>[2x]GPGSNATQINEELYRLLEDTEILNQEITEGLLKGFEVPDAGVAIQLSKRDVVYPARILIIVLSEMWRFGLTKQSESFLAQVLTTIQKVVTQLKGNDLIPSGVFWLANVRELYSFVVFALNS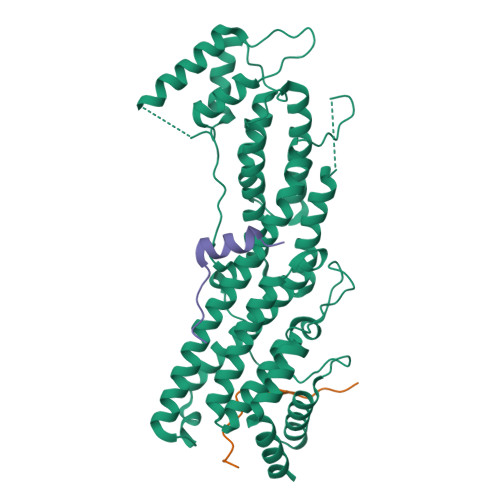ILTEETFKNGMTDEEYKEYVSLVTELKDDFEALSYNIYNIWLKKLQKQLQKKAINAVVISESLPGFSAGETSGANTEEYTMDDILTFFNSIYWCMKSFHIENEVFHAVVTTLLNYVDAICFNELIMKRNFLSWKRGLQLNYNVTRLEEWCKTHGLTDGTECLQHLIQTAKLLQVRKYTIEDIDILRGICYSLTPAQLQKLISQYQVADYESPIPQEILRYVADIVKKEAALSSSGNDSKGHEHSSSIFITPETGPFTDPFSLIKTRKFDQVEAYIPAWLSLPSTKRIVDLVAQQVVQDGH;>[4x]GPGSEFGNSARIPCPKTRLARVSVLDLKKIEEQPDSSSG>[6x]MDHRTSIAQAMVDRISKQMDGSQPDEYFNNLYGNVSRQTYKFEEIREFPYVAVHIGTETGQYLPSGQQWMFLELPILVYDKEKTDIQEQLEKLVADIKTVID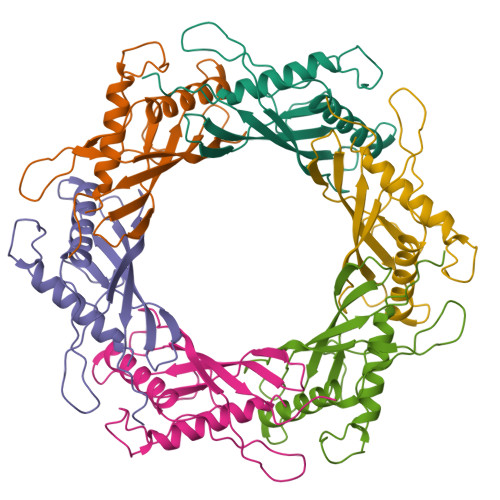TGGNLEYTVSKPNGSTFPCEATDMIITSVSTDEGLLAPYGLAEINVTVRYQPPRRSLRR>[2x]GHGAT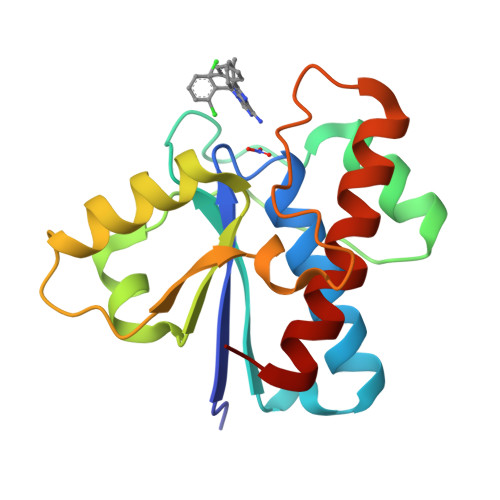KSVLFVCLGNICRSPIAEAVFRKLVTDQNISENWRVDSAATSGYEIGNPPDYRGQSCMKRHGIPMSHVARQITKEDFATFDYILCMDESNLRDLNRKSNQVKTCKAKIELLGSYDPQKQLIIEDPYYGNDSDFETVYQQCVRCCRAFLEKAH> NKALNLQCIKVNNWDLFFSPSEDNFTNDLNKGEEITSDTNIEAAEENISLDLIQQYYLTFNFDNEPENISIENLSSDIIGQLELMPNIERFPNGKKYELDKYTMFHYLRAQEFEHGKSRIALTNSVNEALLNPSRVYTFFSSDYVKKVNKATEAAMFLGWVEQLVYDFTDETSEVSTTDKIADITIIIPYIGPALNIGNMLYKDDFVGALIFSGAVILLEFIPEIAIPVLGTFALVSYIANKVLTVQTIDNALSKRNEKWDEVYKYIVTNWLAKVNTQIDLIRKKMK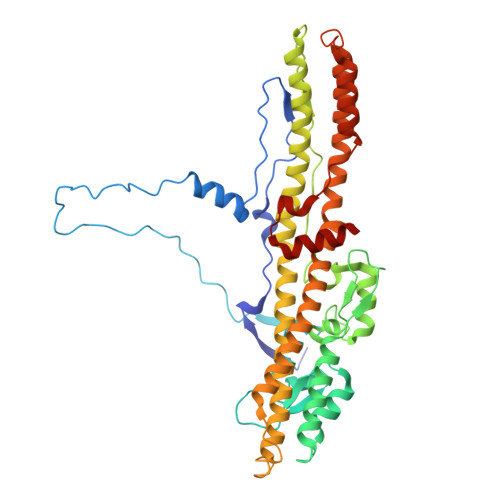EALENQAEATKAIINYQYNQYTEEEKNNINFNIDDLSSKLNESINKAMININKFLNQCSVSYLMNSMIPYGVKRLEDFDASLKDALLKYIYDNRGTLIGQVDRLKDKVNNTLSTDIPFQLSKYVDNQRLLSTFTEYIKNIINTS> SDACVHHIKRRDIVLKWELGEGAFGKVFLAECHNLLPEQDKMLVAVKALKEASESARQDFQREAELLTMLQHQHIVRFFGVCTEGRPLLMVFEYMRHRDLNRFLRSHGPDAKLLAGGEDVAPGPLGLGQLLAVASQVAAGMVYLAGLHFVHRDLATRNC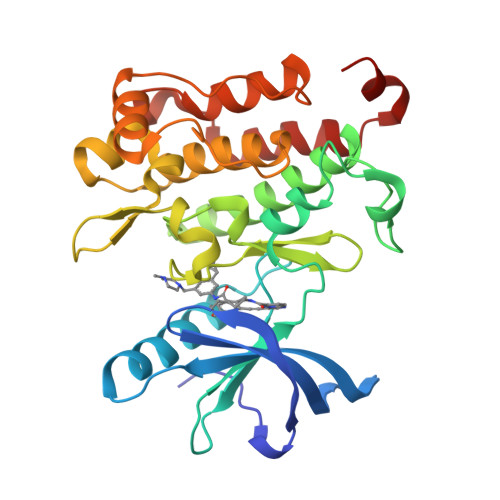LVGQGLVVKIGDFGMSRDIYSTDYYRVGGRTMLPIRWMPPESILYRKFTTESDVWSFGVVLWEIFTYGKQPWYQLSNTEAIDCITQGRELERPRACPPEVYAIMRGCWQREPQQRHSIKDVHARLQALAQAPPVYLDVLG>[8x]MRGSH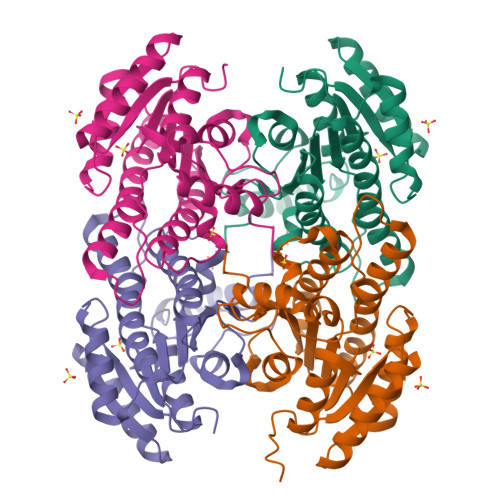HHHHHGSLLIDKTVIVTGASRGIGRAAARECARQGARVVIGHSGSDEGRAGALSLAEEIAAFGGTAIAVGADAADLDSGEKLVAAAVEAFGSVDVLVNNAGICPFHSFLDMPRELYLKTVGTNLNGAYFTVQAAARRMKEQGRGGAIIAVSSISALVGGAMQTHYTPTKAGLLSLMQSCAIALGPYGIRCNAVLPGTIATDINKEDLSDLEKRERMTSRVPLGRLGEPDDLAGPIVFLASDMARYVTGASLLVDGGLFVNLQ(2S)-2-amino-6-[[3-hydroxy-2-methyl-5-(phosphonooxymethyl)pyridin-4-yl]methylideneamino]hexanoic 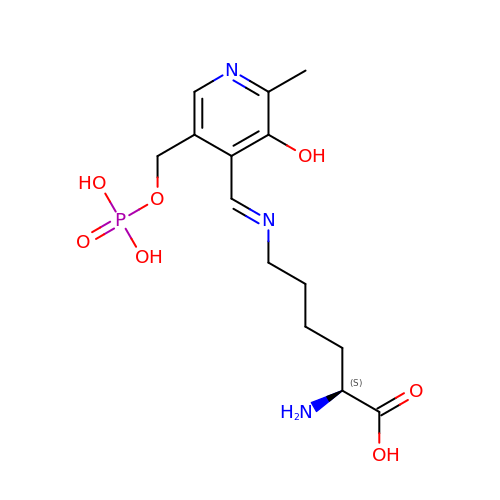acid | C14 H22 N3 O7 P | YQSOQJORMNSDJL-QFULYMJESA-N> TVASISSGPKHTQKVPILTANETGATMPVLPSDSIETRTTYMHFNGSETDVECFLGRAACVHVTEIQNKDATGIDNHREAKLFNDWKINLSSLVQLRKKLELFTYVRFDSEYTILATASQPDSANYSSNLVVQAMYVPPGAPNPKEWDDYTWQSASNPSVFFKVGDTSRFSVPYVGLASAYNCFYDGYSHDDAETQYGITVLNHMGSMAFRIVNE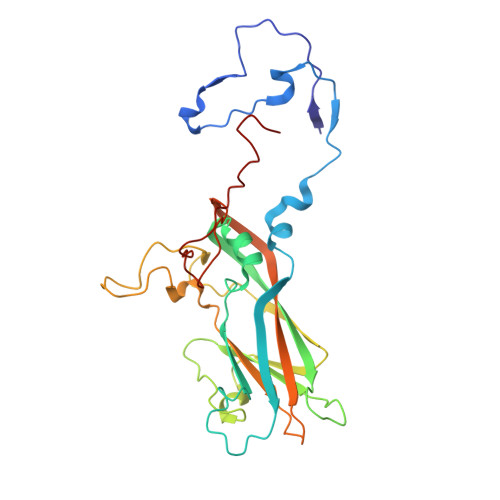HDEHKTLVKIRVYHRAKHVEAWIPRAPRALPYTSIGRTNYPKNTEPVIKKRKGDIKSY>SNAMGEVAYTNGNGNDKSHSPPNGYRKSCWYEEEIEENLRWCFALNSILHTGAS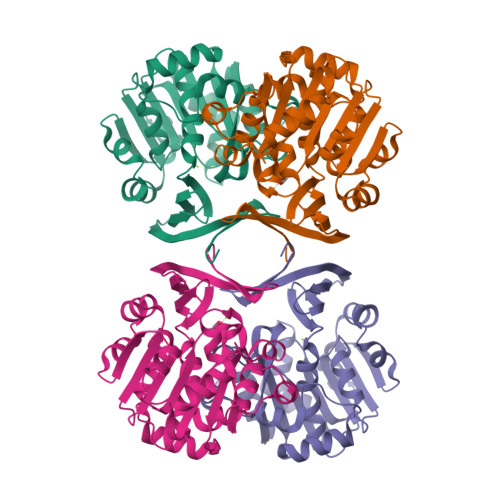QYQDIALLDTKPFGKALVLDGKLQSAETDEFIYHECLVHPALLHHPMPKNVFIMGGGEGSTARELLRHKTIDKVVMCDIDEEVVEFCKSYLVVNKEAFHDSRLEVVINDAKAELEGKEEKYDVIVGDLADPIEGGPCYKLYTKDFYELTLKPKLKKGGIFVTQAGPAGIFSHTEVFSCIYNTLRQVFKYVVPYSAHIPSYADIWGWVLASDSPLDLSAEELDIRMRQRIIEENRYLDGKTFVSSSTLSKAVRNSLNNETHVYTEGAARFIYGHGKNA[2x]>[2x]GDGGGNTQQLSSYAIVDYSSTMRTLIYPLGYYPLYVATIANDPTYRAGDCVLANFTVDFDSADNANASTNGFYVATGAASSPLAKYDLSYSPLDSMALDNELLLSGSESALLFSNN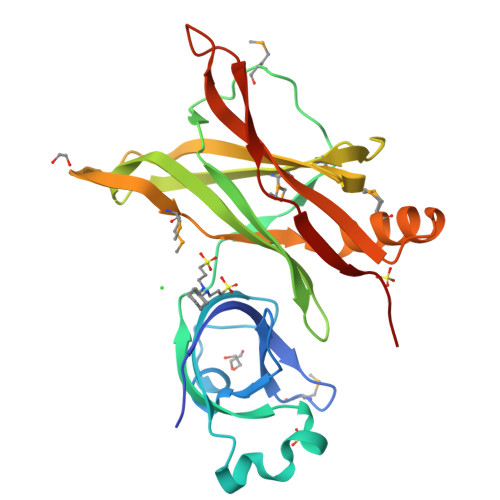YKRIVVIPTFTSVLTDQKNTYIMSMDSNQEPETVDGTDRVYTLCLRAQKREEGKAPTISNAMDPIAVEGGTLYSMLKGKESAAGKKIVSYRVKYPLTFNADSTKIATWGYSKISQFSIEEATN> XQEREV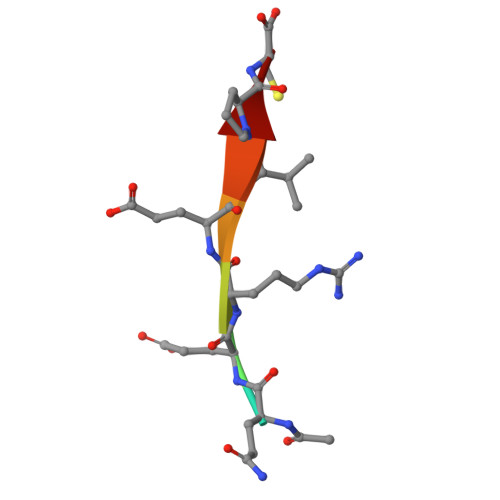PC>[2x]MELSSLTAVSPVDGRYGDKVSALRGIFSEYGLLKFRVQVEVRWLQKLAAHAAIKEVPAFAADAIGYLDAIVASFSEEDAARIKTIERTTNHDVKAVEYFLKEKVAEIPELHAVSEFIHFACTSEDINNLSHALMLKTARDEVILPYWRQLIDGLKDLAVQYRDIPLLSRTNGQPATPSTIGKEMANVAYRMERQYRQLNQVEILGKINGAVGNYNAHIAAYPEVDWHQFSEEFVTSLGIQWNP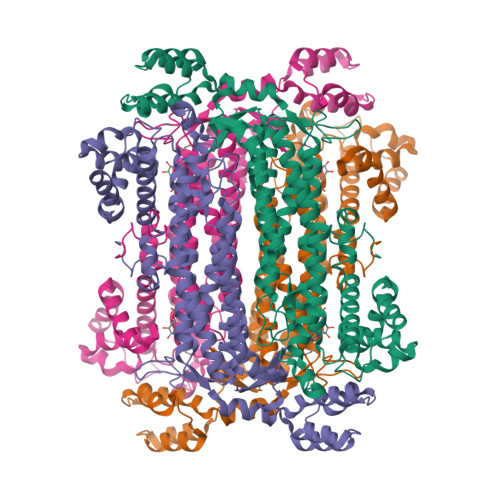YTTQIEPHDYIAELFDCVARFNTILIDFDRDVWGYIALNHFKQKTIAGEIGSSTMPHKVNPIDFENSEGNLGLSNAVLQHLASKLPVSRWQRDLTDSTVLRNLGVGIGYALIAYQSTLKGVSKLEVNRDHLLDELDHNWEVLAEPIQTVMRRYGIEKPYEKLKELTRGKRVDAEGMKQFIDGLALPEEEKARLKAMTPANYIGRAITMVDELKHHHHHH>MGSSHHHHHHSQDPNSNVTLTAVKKAFPDALTNAELVAMVSKRLSQFGYHKYNTLLATSLCSDEVTRPLEQDFGEVYGKHFTMGGLAGFPFGGLTGFGAMAGHIPDGGSCLLIYGSHVGVSWEGKWGTVARRGREKGGACCGSAVAAAQAVTQAYQATLDESSSSSSSSATSTPVYRYSNDPLDAQQGYVRDMLRPYAATLSEAEDVMVTLPVSVYDAQQKLVTRILDEGSNHIDGDGQIAVVGGIQINTPKEMSDFFVVRRFCIRDSSGNMVE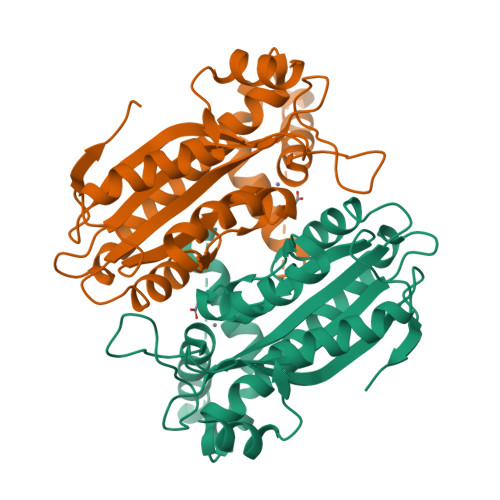NFMPLTAGRE[2x]> GMNLDSYERTGLRVSLDLVNIATPGSRRGTPHTGGCVIEDLHDLLKDDPASVAQLGDDHVEGFVELARLLHTAIDALSNGQVATAATALNHLLRKHPATPELAQDPDGTWRLHHHPLDAELVPMWTAICAEGLAREIGHQNVRRFGICNAHRCDRVYFDTSRNGTRQYCSLACQNRVKAAAFRERRAT

The crystal structure of Jann_2411 from Jannaschia sp. strain CCS1, a member of the Pfam PF07336 family classified as a domain of unknown function (DUF1470), was solved to a resolution of 1.45 Å by multiple-wavelength anomalous dispersion (MAD). This protein is the first structural representative of the DUF1470 Pfam family. Structural analysis revealed a two-domain organization, with the N-terminal domain consisting of a new fold that we call the ABATE (for Alpha-Beta-hairpin-Alpha TandEm) domain and the C-terminal domain forming a treble-clef zinc finger that we have termed the CGNR zinc-finger domain after a characteristic sequence motif that is conserved in this family. Jan_2411 forms a dimer, with both monomers implicated in the formation of a putative DNA binding site, and analysis of its genomic context suggests a role for the ABATE-domain family in stress-induced transcriptional regulation.

The final model included one protomer (residues 1–184), three acetate molecules, two glycerol molecules, one zinc ion, one nickel ion, two sodium ions and 240 water molecules in the asymmetric unit. Arg185, Ala186 and Thr187 at the C-terminus and Gly0 remaining after the cleavage of the expression/purification tag at the N-terminus were disordered and not modeled. The first domain (residues 1–142) can be visualized as two subdomains (H2–H4, β1–β2 and H5–H7, β3–β4) that share similar topology and secondary-structure elements, namely a helix–β-­hairpin–helix motif (H2-β1-β2-H3 in the first subdomain; H6-β3-β4-H7 in the second subdomain), with an additional helix (H4 from the first subdomain and H5 from the second subdomain) linking the two motifs. The helices of the first subdomain (H2 and H3) are stacked per­pendicular to helices H5 and H7 which, together with H6, form a helical bundle capped on one end by the 310-helix H8 and on the other by helix H4. The second domain (residues 143–187; H8, β5–β6, H9) forms a treble-clef zinc finger. A high degree of conservation is observed for a number of positively charged residues (Arg143, Arg161, Arg165, Lys177, Arg182 and Arg184), suggesting that this region could present a nucleic acid binding site. Furthermore, residues 146 (a hydrophobic residue) and 167 (an aromatic residue) are highly conserved and could intercalate between the DNA bases. Analysis of the crystallographic packing of Jann_2411 using the PISA server and analytical size-exclusion chromatography in combination with static light scattering indicate that a dimer is the likely quaternary form. However, given the prediction that the C-terminal domain binds DNA, then the N-­terminal domain may allow the protein to act as a signal-dependent transcriptional regulator with the ABATE domain conferring sensitivity to some as yet undefined ligand.> MSLNDDATFWRNARQHLVRYGGTFEPMIIERAKGSFVYDADGRAILDFTSGQMSAVLGHCHPEIVSVIGEYAGKLDHLFSGMLSRPVVDLATRLANITPPGLDRALLLSTGAESNEAAIRMAKLVTGKYEIVGFAQSWHGMTGAAASATYSAGRKGVGPAAVGSFAIPAPFTYRPRFERNGAYDYLAELDYAFDLIDRQSSGNLAAFIAEPILSSGGIIELPDGYMAALKRKCEARGMLLILDEAQTGVGRTGTMFACQRDGVTPDILTLSKTLGAGLPLAAIVTSAAIEERAHELGYLFYTTHVSDPLPAAVGLRVLDVVQRDGLVARANVMGDRLRRGLLDLMERFDCIGDVRGRGLLLGVEIVKDRRTKEPADGLGAKITRECMNLGLSMNIVQLPGMGGVFRI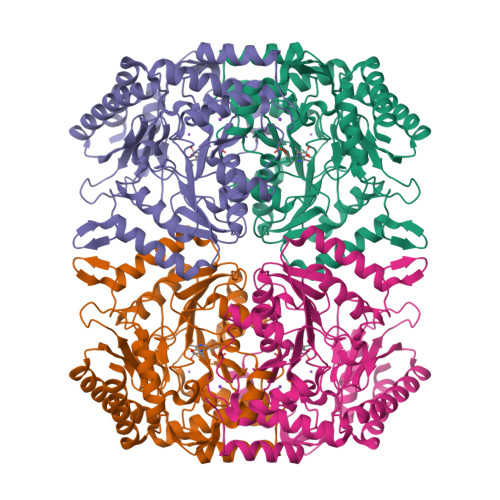APPLTVSEDEIDLGLSLLGQAIERAL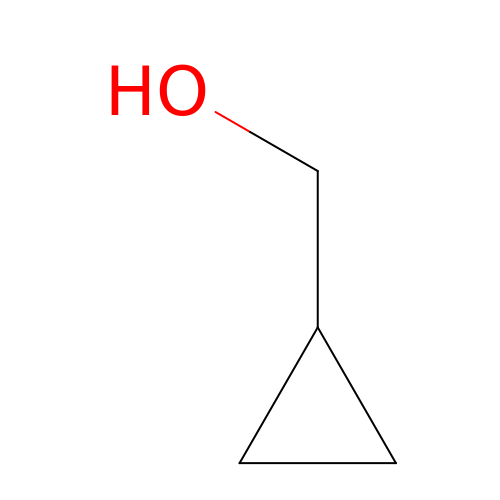cyclopropylmethanol | C4 H8 O | GUDMZGLFZNLYEY-UHFFFAOYSA-N> VETISFSFSEFEPGNDNLTLQGASLITQSGVLQLTKINQNGM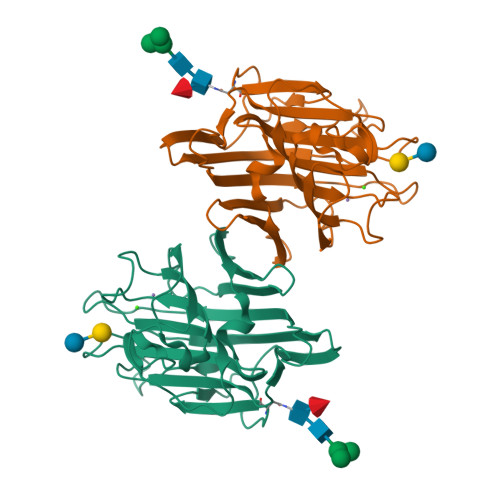PAWDSTGRTLYAKPVHIWDMTTGTVASFETRFSFSIEQPYTRPLPADGLVFFMGPTKSKPAQGYGYLGIFNQSKQDNSYQTLGVEFDTFSNPWDPPQVPHIGIDVNSIRSIKTQPFQLDNGQVANVVIKYDASSKLLHAVLVYPSSGAIYTIAEIVDVKQVLPEWVDVGLSGATGAQRDAAETHDVYSWSFQASLPE dodecyl 2-(trimethylammonio)ethyl phosphate 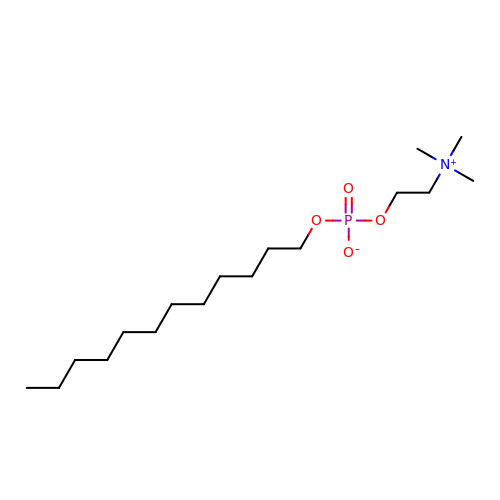| C17 H38 N O4 P | QBHFVMDLPTZDOI-UHFFFAOYSA-N>[16x]ANSHHHHHHGKLTSDFDNPRWIGRHKHMFNFLDVNH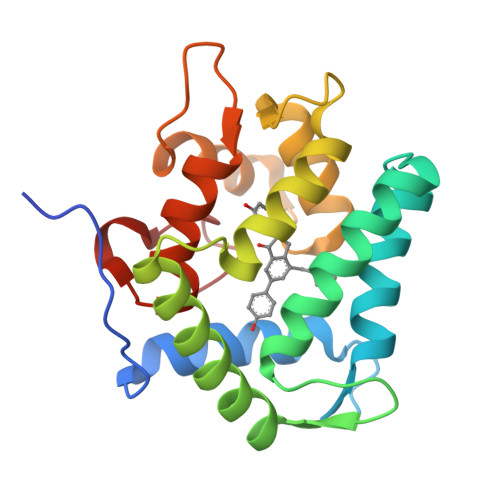NGKISLDEMVYKASDIVINNLGATPEQAKRHKDAVEAFFGGAGMKYGVETDWPAYIEGWKKLATDELEKYAKNEPTLIRIWGDALFDIVDKDQNGAITLDEWKAYTKAAGIIQSSEDCEETFRVCDIDESGQLDVDEMTRQHLGFWYTMDPACEKLYGGAVP> SNTASKSLSPMPQIAGVTYYGDIPKQPKRVVSLASTYTGYLKKLDMNLVGVTSYDKKNPILAKTVKKAKQVAATDLEAITTLKPDLIVVGSTEENIKQLAEIAPVISIEYRKRDYLQVLSDFGRIFNKEGKAKKWLKDW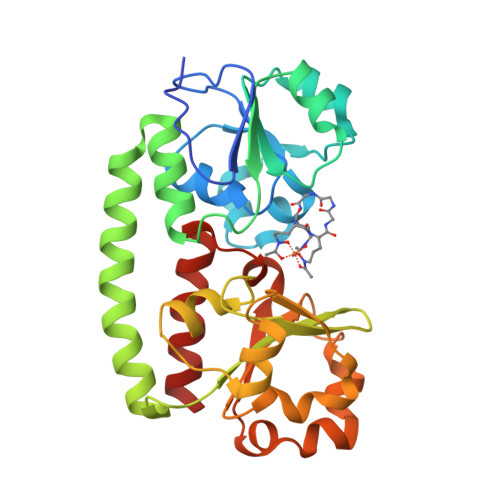KTKTAAYEKEVKAVTGDKATFTIMGLYEKDVYLFGKDWGRGGEIIHQAFHYDAPEKVKTEVFKQGYLSLSQEVLPDYIGDYVVIAAEDDKTGSALYESKLWQSIPAVKKHHVIKVNANVFYFTDPLSLEYQLETLREAILSSEN> TAQTKNTQTLMPLTERVNVQADSARINQIIDGCWVAVGTNKPHAIQRDFTNLFDGKPSYRFELKTEDNTLEGYAKGETKGRAEFSYCYATSDDFRGLPADVYQKAQITKTVYHHGKGACPQGSSRDYEFSVYIPSSLDSNVSTIFAQWHGMPDRTLVQTPQGEVKKLTVDEFVELEKTTFFKKNVGHEKVARLDKQGNPVKDKNGKPVYKAGKPNGWLVEQGGYPPLAFGFSGGLFYIKANSDRKWLTDKDDRCNANPGKTPVMKPLTSEYKASTIAYKLPFADFPKDCWITFRVHIDWTVYGKEAETIVKPGM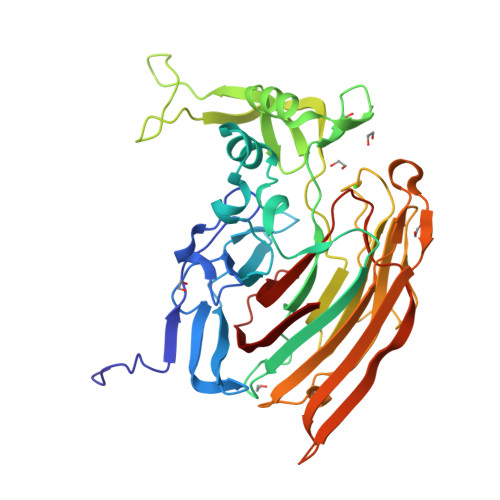LDVRMDYQEQGKKVSKHIVDNEKILIGRNDEDGYYFKFGIYRVGDSTVPVCYNLAGYSER>GQQMGRGSMANSRTVLILCGDYMEDYEVMVPFQALQAFGITVHTVCPGKKAGDSCPTAVHDFCGHQTYFESRGHNFTLNATFDEVDLSKYDGLVIPGGRAPEYLALTASVVELVKEFSRSGKPIASICHGQLILAAADTVNGRKCTAYATVGPSLVAAGAKWVEPITPDVCVVDGSLITAATYEGHPEFIQLFVKALGGKITGANKRILFLCGDYMEDYEVKVPFQSLQALGCQVDAVCPEKKAGDRCPTAIHDFEGDQTYSEKPGHTFALTTNFDDLVSSSYDALVIPGGRAPEYLALNEHVLNIVKEFMNSEKPVASICHGQQILAAAGVLKGRKCTAYPAVKLNVVLGGGTWLEPD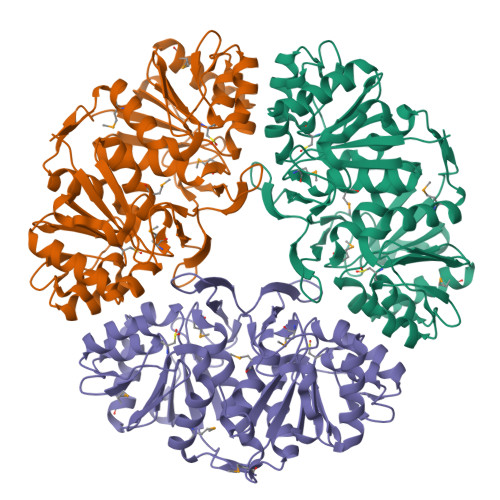PIDRCFTDGNLVTGAAWPGHPEFVSQLMALLGIQVSF[3x]>[4x]UUGC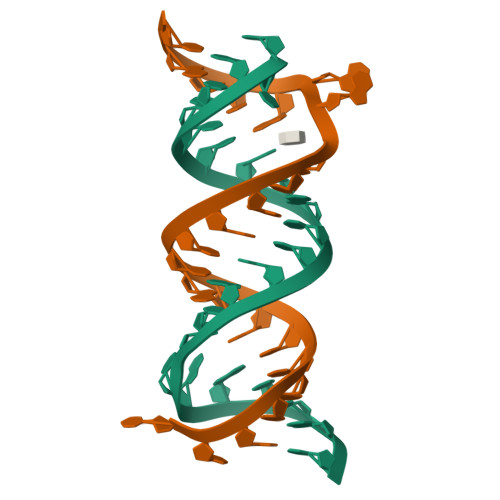GUCACGCCGGCGAAGUCGC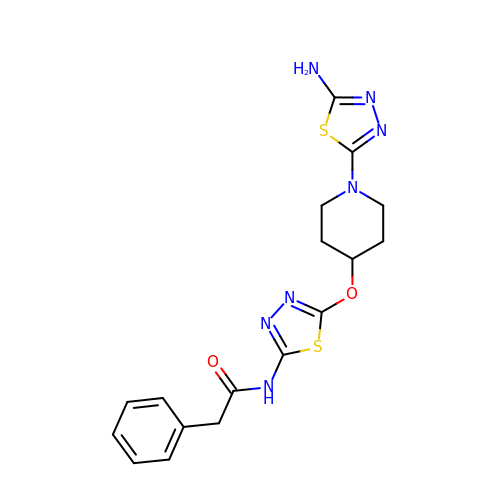N-(5-{[1-(5-amino-1,3,4-thiadiazol-2-yl)piperidin-4-yl]oxy}-1,3,4-thiadiazol-2-yl)-2-phenylacetamide | C17 H19 N7 O2 S2 | KOUAUIYDHAPKFX-UHFFFAOYSA-N> MFHRAFVSSSDLTGCTIALSSVCTQKRYWAKPKKRPKVGQGFHEKAQKWREEYLLDRHRALADSLRAYVEFSTSK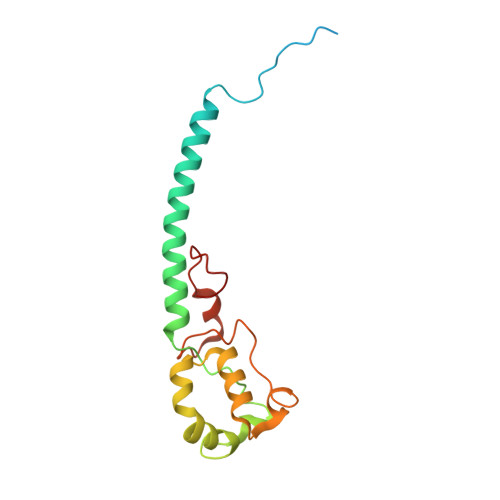RVEPWDARFKPFDRIEKDGVYVLMRYMMEEKLQLCNYHHRPVKRLFCNIGLMGPQITTKARWKPYRFATNPAGTSKAERMYQRDKTVYTHGHND>CTANEQAGKEGSHDKAKTSGEKVLYVNNENEPTSFDPPIGFNNVSWQPLNNIMEGLTRLGKDHEPEPAMAEKWSVSKDNKTYTFTIRENAKWTNGDPVTAGDFEYAWKRMLDPKKGASSAFLGYFIEGGEAYNSGKGKKDDVKVTAKDDRTLEVTLEAPQKYFLSVVSNPAYFPVNEKVDKDNPKWFAESDTFVGNGPFKLTEWKHDDSITMEKSDTYWDKDTVKLDKVKWAMVSDRNTDYQMFQSGELDTAYVPAELSDQLLDQDNVNIVDQAGLYFYRFNVNMEPFQNENIRKAFAMAVDQEEIVKYVTKNNEKPAHAFVSPGFT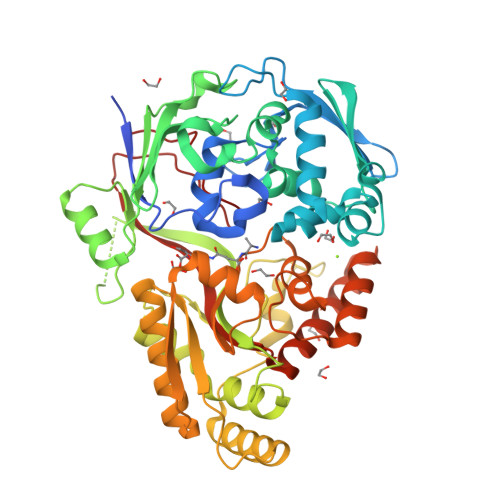QPDGKDFREAGGDLIKPNESKAKQLLEKGMKEENYNKLPAITLTYSTKPEHKKIAEAIQQKLKNSLGVDVKLANMEWNVFLEDQKALKFQFSQSSFLPDYADPISFLEAFQTGNSMNRTGWANKEYDQLIKQAKNEADEKTRFSLMHQAEELLINEAPIIPVYFYNQVHLQNEQVKGIVRHPVGYIDLKWADKN[3x]> DNGCSVAAESTNFTVDLMENAAKQFNNIGATTPVVPFRILLSPCGNAVSAVKVGFTGVADSHNANLLALENTVSAASGLGIQLLNEQQNQIPLNAPSSALSWTTLTPGKPNTLNFYARLMATQVPVTAGHINATAT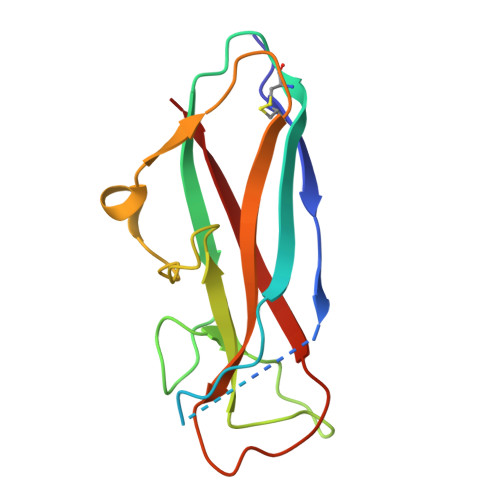FTLEYQ>[4x]MSKKQKSKYIVIFGCGRLGSLIANLASSSGHSVVVVDKNEYAFHRLNSEFSGFTVVGDAAEFETLKECGMEKADMVFAFTNDDSTNFFISMNARYMFNVENVIARVYDPEKIKIFEENGIKTICPAVLMIEKVKEFIIGSEED;>MKVIIIGGETTAYYLARSMLSRKYGVVIINKDRELCEEFAKKLKATIIHGDGSHKEILRDAE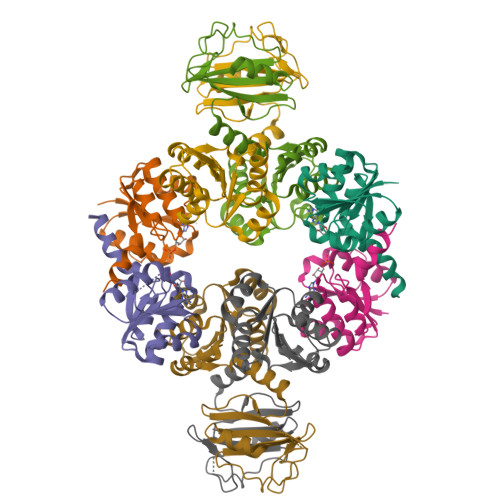VSKNDVVVILTPRDEVNLFIAQLVMKDFGVKRVVSLVNDPGNMEIFKKMGITTVLNLTTLITNTVEALIFPDEFSSIIPLEQGIEFLSVNVEEDSPVVGKKLKDLPLPRDSIIAAIVRGGVLVVPRGDTEILSGDKLYVIVSAEAKETVEETLLGR[4x]>MEPTTEIQATEDLTLSGDHAAASADSLVVDNANDNAGQEEGFEIVLKDDETAPKQDPAKNAEFARRRIERKRQRELEQQMEAVKRGELPESLRVNPDLPPQPDINAYLSEEGLAKYDYDNSRALAAFNAANTEWLMKAQDARSNAVAEQGRKTQEFTQQSAQYVEAARKHYDAAEKLNIPDYQEKEDAFMQLVPPAVGADIMRLFPEKSAALMYHLGANPEKARQLLAMDGQSALIELTRLSERLTLKPRGKQISSAPPADQPITGDVSAANKDAIRKQMDAAASKGDVETYRKLKAKLKGIR[3x]

Tailed double-stranded DNA (dsDNA) bacteriophages and their eukaryotic counterparts, such as herpesviruses, possess a dodecameric portal at a unique vertex of the capsid; this portal serves as a channel for DNA packaging during viral assembly and delivery. The portal interacts with multiple copies of a scaffolding protein (SP) to form a nucleation complex, which initiates the assembly of the major capsid protein (i.e., coat protein) and other minor proteins into a procapsid. The P22 procapsid consists of an icosahedral coat comprising 415 coat protein (gene product [gp] 5) subunits, a dodecameric ring comprising portal protein (gp1) subunits located at a unique capsid vertex, and an internal core comprising approximately 250–300 SP (gp8) subunits and 3 ejection proteins. In this study, we present the structure of the SP gp8 in complex with the dodecameric portal in the P22 procapsid at subnanometer resolution.

Three column-like structures, each interacting with two neighboring nodules, were observed on the GOF nodules. The nine nodules, which were essentially identical, were formed by α-helices, and each column was formed by a three-helix bundle. On each GOF, each column connecting two neighboring nodules consisted of a three-helix bundle. The three α-helices were contributed by the column domains of the inner base-associated gp8, the outer base-associated gp8 from the neighboring nodule, and the side nodule-associated gp8. These three SP subunits interacted through the three-helix bundle, forming an SP trimer. The gp8 subunits interacted with the neighboring portal subunits. Each trimer interacts with two neighboring portal subunits.> MASMTGGQQMGRGSMKFLFYLSADNLEIARKEVLVLAERYGWVEDYQFEERLLLLDYAGEKFFERLAYTNEVTKIYDICSVSELEQVFSEIPVYDRLCCVRVKGGKGKTALERKLGALLWKRGAKVSVSNPEIVYKVYIQDDKCYVGLLEFERDTRQFFLRRPDRRPFLMPSAIKPKLARALVNLTGVLEGETLLDPMCGTGSFLIEAGLMGINPIGIDFIEKIVRGCRVNLEYYGIEGSVLLGDAKNLPLRDESVRGIA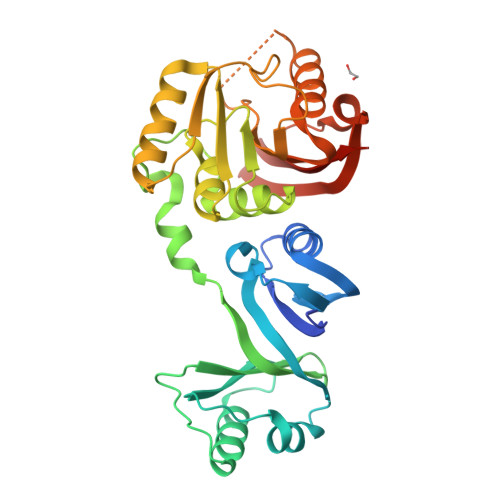TDYPYLRSTKAAGTLDELYSKTSEEFERVLKKGGRAAIVTNIDVESFFSNFEIEMKTEERVHGSLTRRIYLLRRHHHHHH>NNTLWTGPKPEANCIIEYGKQNPDSKLTLILVKNGGIVNGYVTLMGASDYVNTLFKNKNVSINVELYFDATGHILPDSSSLKTDLELKYKQTADFSARGFMPSTTAYPFVLPNAGTHNENYIFGQCYYKASDGALFPLEVTVMLNKRLPDSRTSYVMTFLWSLNAGLAPETTQATLITSPFTFSYIRED[3x];>[2x]PVFTQDVFVGSVEELSAAHTLVMKINATDADEPNTLNSKISYRIVSLEPAYPPVFYLNKDTGEIYTTSVTLDREEHSSYTLTVEARDGNGEVTDKPVKQAQVQIRILDVNDNIPVVENKVLEGMVEENQVNVEVTRIKVFDADEIGSDNWLANFTFASGNEGGYFHIETDAQTNEGIVTLIKEVDYEEMKNLDFSVIVANKAA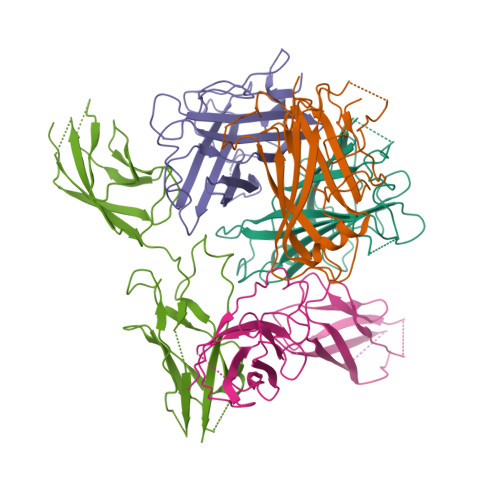FHKSIRSKYKPTPIPIKVKVK> MLKQVEIFTDGSCLGNPGPGGYGAILRYRGREKTF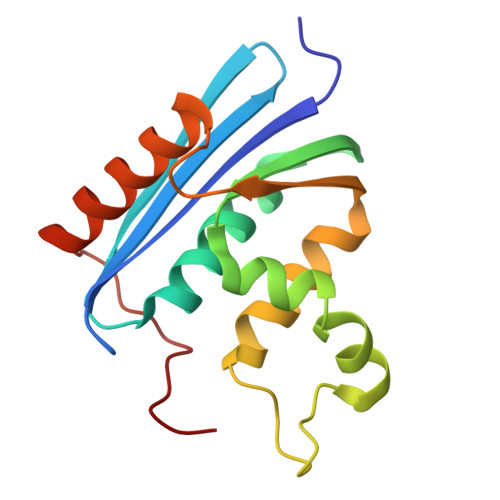SAGYTRTTNNRMELMAAIVALEALKEHCEVILSTDSQYLRQGITQWIHNWKKRGWKTADKKPVKNVDLWQRLDAALGQHQIKWEWVKGHAGHPENERCDELARAAAMNPTLEDTGYQVEV methyl 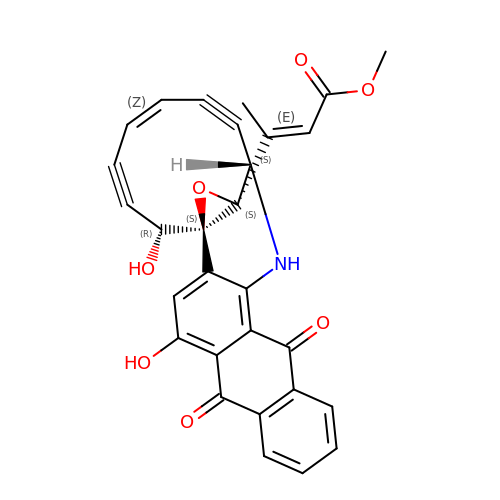(2E)-3-[(1aS,11S,11aS,14Z,18R)-3,18-dihydroxy-4,9-dioxo-4,9,10,11-tetrahydro-11aH-11,1a-hept[3]ene[1,5]diynonaphtho[2,3-h]oxireno[c]quinolin-11a-yl]but-2-enoate | C29 H19 N O7 | VNWTWPJYWHYMNF-PUHZCEAISA-N> MAKGGFNLSDWALRHQSLVWYLMAVSLVMGVFSYLNLGREEDPSFAIKTMVIQTRWPGATVDDTLEQVTDRIEKKLEELDSLDYVKSYTRPGESTVFVYLKDTTKAGDIPDIWYQVRKKISDIQGEFPQGIQGPGFNDEFGDVFGSVYAFTADGLDFRQLRDYVEKVRLDIRSVKDLGKVQMIGAQNEVIYLNFSTRKLAALGLDQRQVVQSLQAQNAVTPSGVVEAGPERISVRTSGNFRSEKDLQAVNLRVNDRFYRLSDLASISRDFVDPPTSLFRYKGEPAIGLAVAMKEGGNI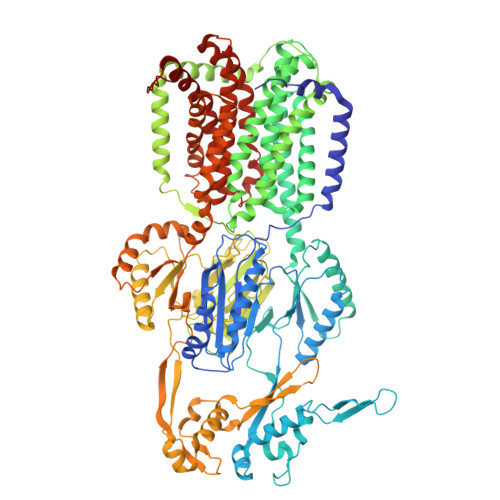LEFGEALNARMQEITGELPVGVGVHQVSNQAQVVKKAVGGFTRALFEAVVIVLIVSFVSLGLRAGLVVACSIPLVLAMVFVFMEYTDITMQRVSLGALIIALGLLVDDAMITVEMMITRLELGDSLHDSATYAYTSTAFPMLTGTLVTVAGFVPIGLNASSAGEYTFTLFAVIAVALLLSWIVAVLFAPVIAVHILPKTLKHKSEQKKGRIAERFDSLLHLAMRRRWTTIFLTALLFGVSLFLMKFVQHQFFPSSDRPELLVDLNLPQNSSIHETRAVMDRLEATLKDDEDIDHWSAYVGEGAIRFYLPLDQQLQNNFYGQLVIVTKDLEARERVAARLRDRLRKDYVGISTYVQPLEMGPPVGRPIQYRVSGPQIDKVREYAMGLAGVLDGNPNIGDIVYDWNEPGKMLKIDIAQDKARQLGLSSEDVAQIMNSVVTGSAVTQVRDDIYLVNVIGRAEDSERGSLETLESLQIVTPSGTSIPLKAFAKVSYELEQPLVWRRDRKPTITVKASLRGEIQPTDLVARLAPEVKRFADGLPANYRIEVGGTVEESGKAEGPIAKVVPLMLFLMATFLMIQLQSVQKLFLVASVAPLGLIGVVAALLPTGTPMGFVAILGILALIGIIIRNSVILVTQIDAFEKDGKTPWEAVLEATHHRTRPILLTAAAASLGMIPIAREVFWGPMAYAMIGGIVAATLLTLIFLPALYVAWYRIPEPGRHHHHHH>MGGSHHHHHHRSESTVTEELKEGIDAVYPSLVGTADSKAEGIKNYFKLSFTLPEEQKSRTVGSEAPLKDVAQALSSRARYELFTEKETANPAFNGEVIKRYKELMEHGEGIADILRSRLAKFLNTKDVGKRFAQGTEANRWVGGKLLNIVEQDGDTFKYNEQLLQTAVLAGLQWRLTATSNTAIKDAKDVAAITGIDQALLPEGLVEQFDTGMTLTEAVSSLAQKIESYWGLSRNPNAPLGYTKGIPTAMAAEILAAFVESTDVVENIVDMSEIDPDNKKTIGLYTITELDSFDPINSFPTAIEEAVLVNPTEKMFFGDDIPPVANTQLRNPAVRNTPEQKAALKAEQATEFYVHTPMVQFYETLGKDRILELMGAGTLNKELLNDNHAKSLEGKNRSVEDSYNQLFSVIEQVRAQSEDISTVPIHYAYNMTRVGRMQMLGKYNPQSAKLVREAILPTKATLDLSNQNNEDFSAFQLGLAQALDIKVHTMTREVMSDELTKLLEGNLKPAIDMMVEFNTTGSLPENAVDVLNTALGDRKSFVALMALMEYSRYLVAEDKSAFVTPLYVEADGVTNGPINAMMLMTGGLFTPDWIRNIAKGGLFIGSPNKTMNEHRSTADNNDLYQASTNALMESLGKLRSNYASNMPIQSQIDSLLSLMDLFLPDINLGENGALEL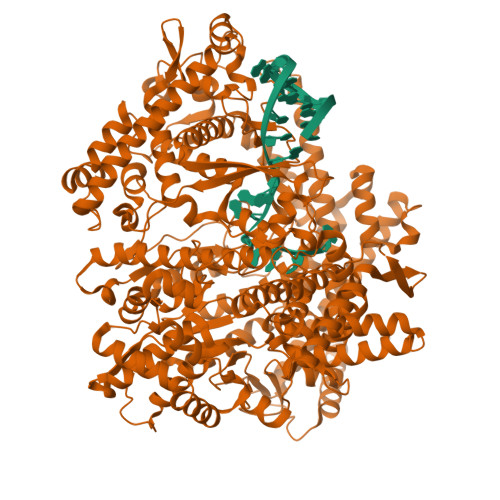KRGIAKNPLTITIYGSGARGIAGKLVSSVTDAIYERMSDVLKARAKDPNISAAMAMFGKQAASEAHAEELLARFLKDMETLTSTVPVKRKGVLELQSTGTGAKGKINPKTYTIKGEQLKALQENMLHFFVEPLRNGITQTVGESLVYSTEQLQKATQIQSVVLEDMFKQRVQEKLAEKAKDPTWKKGDFLTQKELNDIQASLNNLAPMIETGSQTFYIAGSENAEVANQVLATNLDDRMRVPMSIYAPAQAGVAGIPFMTIGTGDGMMMQTLSTMKGAPKNTLKIFDGMNIGLNDITDASRKANEAVYTSWQGNPIKNVYESYAKFMKNVDFSKLSPEALEAIGKSALEYDQRENATVDDIANAASLIERNLRNIALGVDIRHKVLDKVNLSIDQMAAVGAPYQNNGKIDLSNMTPEQQADELNKLFREELEARKQKVAKA[2x]methyl (4-{6-[(1S)-2-[(3R)-1-acetylpiperidin-3-yl]-1-({(2E)-3-[5-chloro-2-(1H-tetrazol-1-yl)phenyl]prop-2-enoyl}amino)ethyl]-3-chloropyridazin-4-yl}phenyl)carbamate 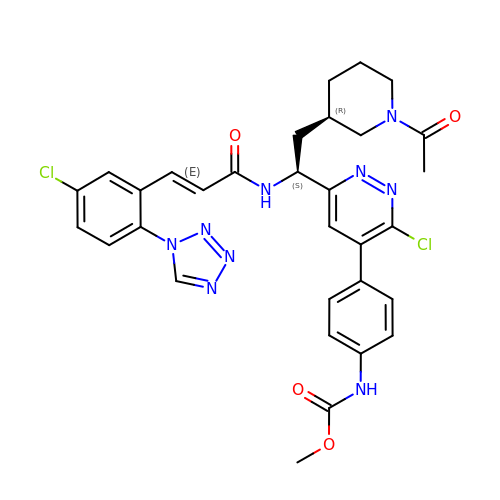| C31 H31 Cl2 N9 O4 | QCCGVMDYTWPPFU-BONIYOLGSA-N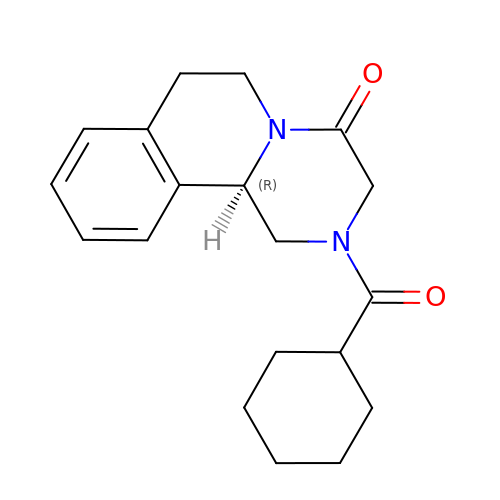PRAZIQUANTEL | C19 H24 N2 O2 | FSVJFNAIGNNGKK-KRWDZBQOSA-N> GSYDYLFKVVLIGDSGVGKSNLLSRFTRNEFNLESKSTIGVEFATRSIQVDGKTIKAQIWDTAGQERYRAITSAYYRGAVGALLVYDIAKHLTYENVERWLKELRDHADSNIVIMLVGNKSDLRHLRAVPTDEARAFAEKNNLSFIETSALDSTNVEEAFKNILTEIYRIVSQKQIADRAAHDESPGNNVVDISVPP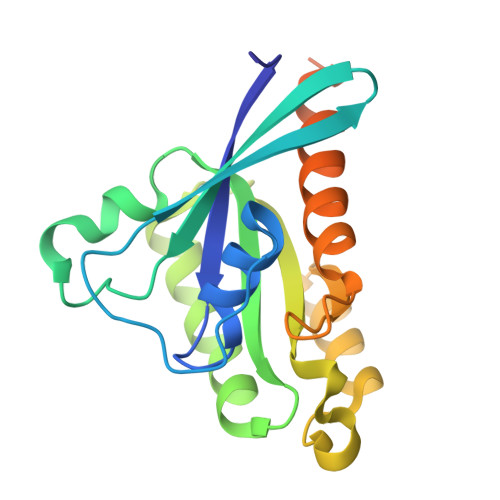TTD> GGGRMEHVDSDFAPIRRSKKVVDSDKIVKAISDDLEQKNFTVLRKLNLVPIKKSVSSPKVCKPSPVKERVDHVFYQKFKSMALQELGTNYLSISYVPSLSKFLSKNLRSMKNCIVFFDKVEHIHQ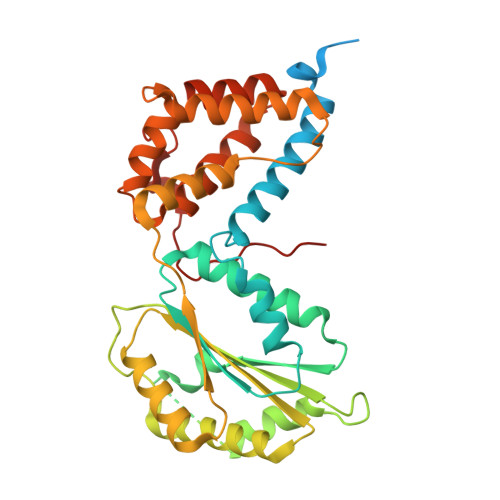YAGIDRAVSETLSLVDINVVIIEMNDYLMKEGIQSSKSKECIESMGQASYSGQLDFEASEKPSNHTSDLMMMVMRKINNDESIDHIVYFKFEQLDKLSTSTIIEPSKLTEFINVLSVLEKSNNIAFKVLIYSNNVSISSLLSTSLKKKLNTKYTVFEMPILTCAQEQEYLKKMIKFTFDSGSKLLQSYNSLVTCQLNNKESNLAIFFEFLKVFPHPFTYLFNAYTEIIVQSRTFDELLDKIRNRLTIKNYPHSAYNFKKNQRLPLKLTRKVHDR> NLDCWVDNEEDIDVILKKSTILNLDINNDIISDISGFNSSVITYPDAQLVPGINGKAIHLVNNESSEVIVHKAMDIEYNDMFNNFTVSFWLRVPKVSASHLEQYGTNEYSIISSMKKHSLSIGSGWSVSLKGNNLIWTLKDSAGEVRQITFRDLPDKFNAYLANKWVFITITNDRLSSANLYINGVLMGSAEITGLGAIREDNNITLKLDRCNNNNQYVSIDKFRIFCKALNPKEIEKLYTSYLSITFLRDFWGNPLRYDTEYYLIPVASSSKDVQLKNITDYMYLTNAPSYTNGKLNIYYRRLYNGLKFIIKRYTPNNEIDSFVKSGDFIKLYVSYNNNEHIVGYPKDGNAFNNLDRILRVGYNA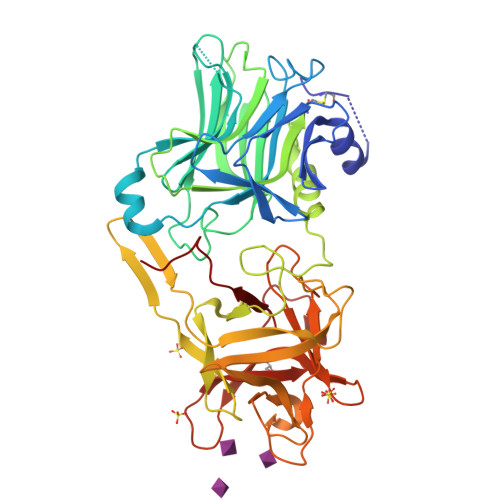PGIPLYKKMEAVKLRDLKTYSVQLKLYDDKNASLGLVGTHNGQIGNDPNRDILIASNWYFNHLKDKILGCDWYFVPTDEGWTND>[2x]MMMKISFIIATLNSGGAERVLVTLANALCKEHEVSIIKFHTGESFYKLENEVKVTSLEQFRFDTLYHKIASRFKKFFALRKALKESKADVFISFLDTTNIACILANIGLKTPLIISEHSNEAYLKPKTWRFLRRVSYPFCDALSVLGSSDKVYYERFVKRVKLLLN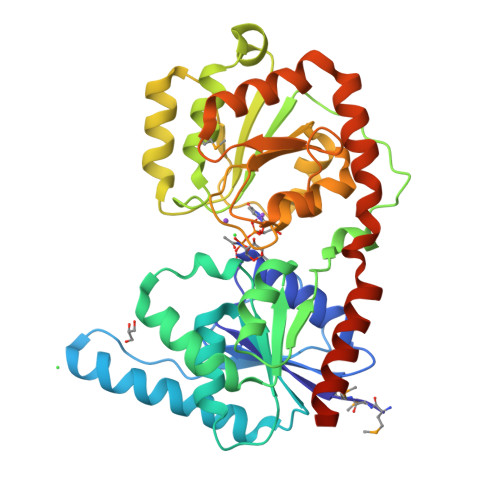PCHFSDEIPFDSSFEKENLVLFIGRLDHNKNPVMFLKAIAHLDKNLQENYKFVIAGDGELRQELEYKVKSLGIKVDFLGRVENVKALYEKAKVLCLCSFVEGLPTVLIESLYFEVCRISSSYYNGAKDLIKDNHDGLLVGCDDEIALAKKLELVLNDENFRKELVNNAKQRCKDFEISNIKEEWLKLIVEVKNALGSHHHHHHHHHH>MEDPLIGRDSLGGGGTDRVRRSEAITHGTPFQKAAALVDLAEDGIGLPVEILDQSSFGESARYYFIFTRLDLIWSLNYFALLFLNFFEQPLWCEKNPKPSCKDRDYYYLGELPYLTNAESIIYEVITLAILLVHTFFPISYEGSRIFWTSRLNLVKVACVVILFVDVLVDFLYLSPLAFDFLPFRIAPYVRVIIFILSIRELRDTLVLLSGMLGTYLNILALWMLFLLFASWIAFVMFEDTQQGLTVFTSYGATLYQMFILFTTSNNPDVWIPAYKSSRWSSVFFVLYVLIGVYFVTNLILAVVYDSFKEQLAKQVSGMDQMKRRMLEKAFGLIDSDKNGEIDKNQCIKLFEQLTNYRTLPKISKEEFGLIFDELDDTRDFKINKDEFADLCQAIALRFQKEEVPSLFEH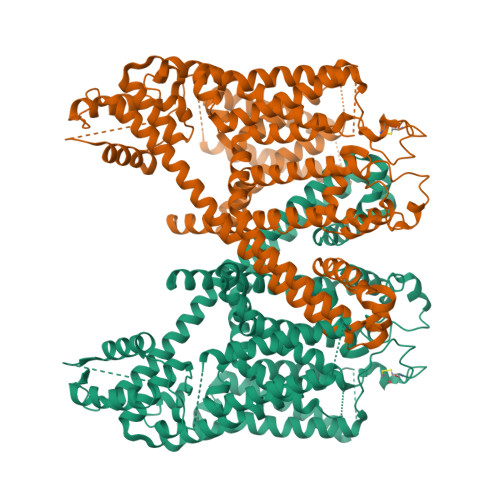FPQIYHSALSQQLRAFVRSPNFGYAISFILIINFIAVVVETTLNIEESSAQKPWQVAEFVFGWIYVLEMALKIYTYGFENYWREGANRFDFLVTWVIVIGETATFITPDENTFFSNGEWIRYLLLARMLRLIRLLMNVQRYRAFIATFITLIPSLMPYLGTIFCVLCIYCSIGVQVFGGLVNAGNKKLFETELAEDDYLLFNFNDYPNGMVTLFNLLVMGNWQVWMESYKDLTGTWWSITYFVSFYVITILLLLNLVVAFVLEAFFTELDLEEEEKCQGQDSQEKRNRRRSAGSKSRSQRVDTLLHHMLGDELSKPECSTSDT[2x]>[4x]SNAMFSAKKLSPADKLKNISSMLEEIVEDTT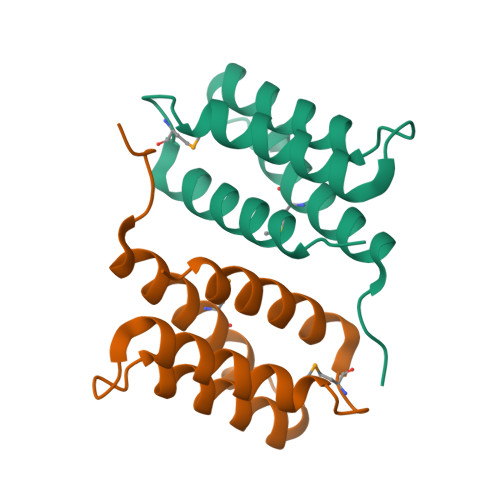VPRNIRAAADNAKNALHNEEQELIVRSATAIQYLDDISEDPNMPIHTRTQIWGIVSELETIKN> WNNIVFYSLGDVNSY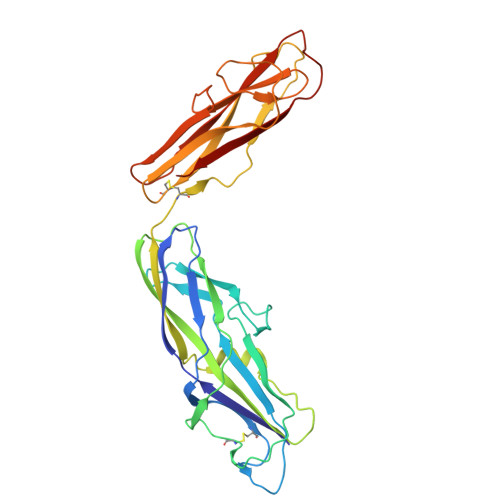QGGNVVITQRPQFITSWRPGIATVTWNQCNGPEFADGFWAYYREYIAWVVFPKKVMTQNGYPLFIEVHNKGSWSEENTGDNDSYFFLKGYKWDERAFDAGNLCQKPGEITRLTEKFDDIIFKVALPADLPLGDYSVKIPYTSGMQRHFASYLGARFKIPYNVAKTLPRENEMLFLFKNIGGCRPSAQSLEIKHGDLSINSANNHYAAQTLSVSCDVPANIRFMLLRNTTPTYSHGKKFSVGLGHGWDSIVSVNGVDTGETTMRWYKAGTQNLTIGSRLYGESSKIQPGVLSGSATLLMILP>[2x]AEQKTLHIYNWTDYIAPDTVANFEKETGIKVVYDVFDSNEVLEGKLMAGSTGFDLVVPSAYALERQLTAGVFQPLDKSKLPEWKNLDPELLKLVAKHDPDNKFAMPYMWATTGIGYNVDKVKAVLGENAPVDSWDLILKPENLEKLKSCGVSFLDDPEEVFATVLNYLGKDPNSTKADDYTGPATDLLLKLRPNIRYFHSSQYINDLANGDICVAIGWAGDVWQ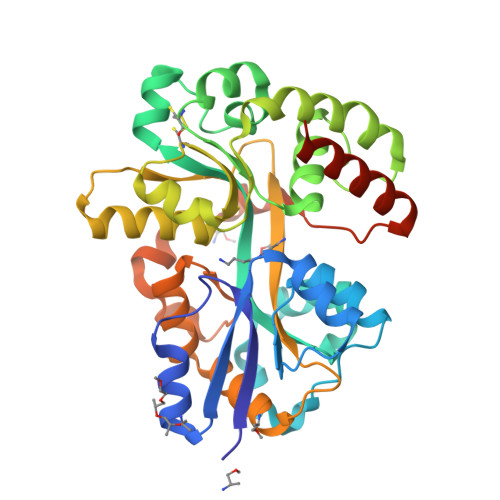ASNRAKEAKNGVNVSFSIPKEGAMAWFDVFAMPADAKNKDEAYQFLNYLLRPDVVAHISDHVFYANANKAATPLVSAEVRENPGIYPPADVRAKLFTQKVQDPKIDRVRTRAWTKVKSGKLEHHHHHH>EDILPCVPFSVAKSVKSLYLGRMFSGTPVIRLRFKRLQPTRLVAEFDFRTFDPEGILLFAGGHQDSTWIVLALRAGRLELQLRYNGVGRVTSSGPVINHGMWQTISVEELARNLVIKVNRDAVMKIAVAGDLFQPERGLYHLNLTVGGIPFHEKDLVQPINPRLDGCMRSWNWLNGEDTTIQETVKVNTRMQCFSVTERGSFYPGSGFAFYSLDYMRTPLDVGTESTWEVEVVAHIRPAADTGVLFALWAPDLRAVPLSVALVDYHSTKKLKKQLVVLAVEHTALALMEIKVCDGQEHVVTVSLRDGEATLEVDGTRGQSEVSAAQLQERLAVLERHLRSPVLTFAGGLPDVPVTSAPVTAFYRGCMTLEVNRRLLDLDEAAYKHSDITAHSCPPVEPAAA[2x];>EESPFVSNPGNITGARGLTGTLRCQLQVQGEPPEVHWLRDGQILELADSTQTQVPLGEDEQGDWIVASQLRITSLQLSDTGQYQCLVFLGHQTFVSQPGYVRLEGLPYFLEEPEDRTVAANTPFNLSCQAQGPPEPVDLLWLQDAVPLATAPGHGPQRSLHVPGLNKTS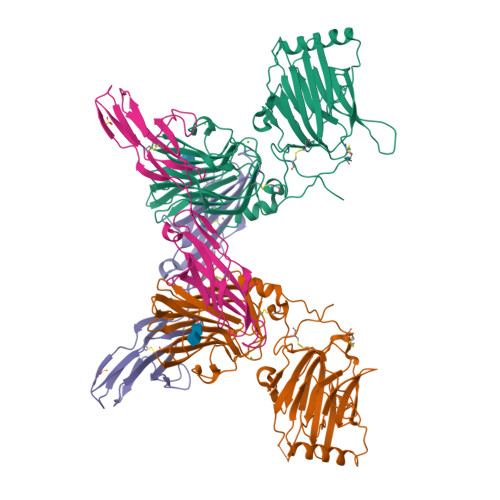SFSCEAHNAKGVTTSRTATITVLPQQ[2x]> LEL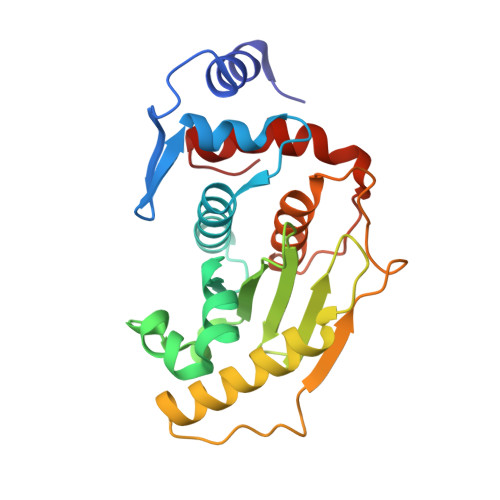TEDMEKEISNALGHGPQDEILSSAFKLRITRGDIQTLKNYHWLNDEVINFYMNLLVERNKKQGYPALHVFSTFFYPKLKSGGYQAVKRWTKGVNLFEQEIILVPIHRKVHWSLVVIDLRKKCLKYLDSMGQKGHRICEILLQYLQDESKTKRNSDLNLLEWTHHSMKPHEIPQQLNGSDSGMFTCKYADYISRDKPITFTQHQMPLFRKKMVWEILHQQLL>GXGTACGC[2x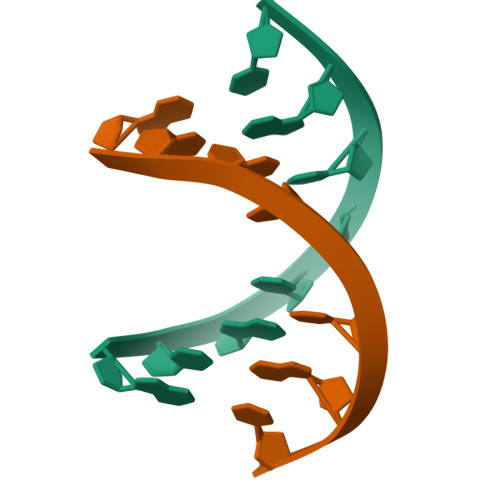]We sought to use our protocol to design a human transferrin receptor (hTfR) binding protein. hTfR transports transferrin (the major carrier of iron in the body) across the blood–brain barrier (BBB) via receptor mediated transcytosis, and this process has been exploited to deliver therapeutic payloads into the brain parenchyma that would otherwise be blocked by the BBB. We developed a computational design approach for designing binding proteins with beta sheets geometrically poised to pair with exposed beta strands in target proteins of interest. We targeted the region surrounding an edge strand located in the hTfR apical domain. This domain is distant from the transferrin binding site (which is important to avoid competitive binding) and is exposed and therefore suitable for beta sheet extension.

However, for strategy 2, one design (designated 2DS25) clearly bound fluorescently labeled hTfR. In the 2DS25 design model, two helices on either side of the central beta sheet extension make contacts with TfR across the interface. To probe the sequence determinants of folding and binding, and to facilitate determination of the structure of the 2DS25–hTfR complex, we created a site saturation mutagenesis (SSM) library in which each position on 2DS25 was substituted with all other 20 amino acids one at a time and screened for hTfR binding using fluorescence-activated cell sorting. The key interface residues were also conserved, while affinity-increasing substitutions were identified around the interface. Combination of these enriched substitutions yielded higher affinity variants. The crystal structures of two increased affinity variants (2DS25.1 and 2DS25.5) in complex with hTfR were determined to be resolutions of 3.1 and 2.8 Å, respectively. The structures are virtually identical with an rmsd of 0.26 Å. In both cases, the design binds the Apical domain of hTfR using beta sheet extension and overall closely resembles the computational design model. The structure of 2DS25 superimposes closely on the computational model with an rmsd of 1.2 Å; this is notable as the fold is more complex than that of previous computationally designed binders. The structural differences in the receptor are at both the backbone and side chain level, in particular at Tyr211; a superposition of all hTfR apo and holo structures in the PDB shows this region is flexible and can exist in multiple conformations.

>RLYWDDLKRKLSEKLDSTDFTSTIKLLNENSYVPREAGSQKDENLALYVENQFREFKLSKVWRDQHFVKIQVKDSAQNSVIIVDKNGRLVYLVENPGGYVAYSKAATVTGKLVHANFGTKKDFEDLYTPVNGSIVIVRAGKITFAEKVANAESLNAIGVLIYMDQTKFPIVNAELSFFGHAHLGTGDPYTPGFPSFNHTQFPPSRSSGLPNIPVQTISRAAAEKLFGNMEGDCPSDWKTDSTCRMVTSESKNVKLTVSNVLKEIKILNIFGVIKGFVEPDHYVVVGAQRDAWGPGAAKSGVGTALLLKLAQMFSDMVLKDGFQPSRSIIFASWSAGDFGSVGATEWLEGYLSSLHLKAFTYINLDKAVLGTSNFKVSASPLLYTLIEKTMQNVKHPVTGQFLYQDSNWASKVEKLTLDNAAFPFLAYSGIPAVSFCFCEDTDYPYLGTTMDTYKELIERIPELNKVARAAAEVAGQFVIKLTHDVELNLDYERYNSQLLSFVRDLNQYRADIKEMGLSLQWLYSARGDFFRATSRLTTDFGNAEKTDRFVMKKLNDRVMRVEYHFLSPYVSPKESPFRHVFWGSGSHTLPALLENLKLRKQNNGAFNETLFRNQLALATWTIQGAANALSGDVWDIDNEF[2x];>[2x]DEEEIQKAIEELLRKGVSEEEAAIIIVQRFNVAVVVVVQDERQAKHISEYIRRYIPEADVILFANIVVIKVETHELRKRVWEAAQKAY>[2x]TETTSFLITKFSPDQQNLIFQGDGYTTKEKLTLTKAVKNTVGRALYSSPIHIWDRETGNVANFVTSFTFVINAPNSYNVADGFTFFIAP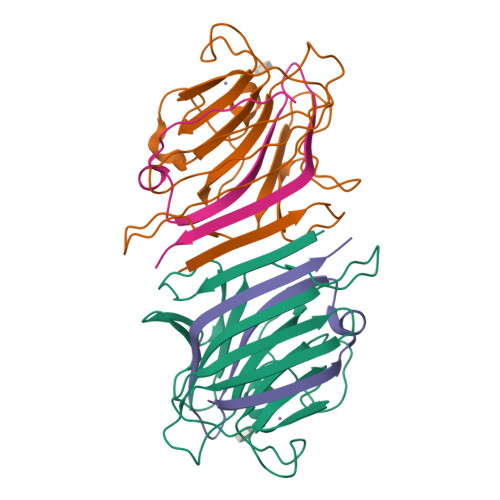VDTKPQTGGGYLGVFNSAEYDKTTQTVAVEFDTFYNAAWDPSNRDRHIGIDVNSIKSVNTKSWKLQNGEEANVVIAFNAATNVLTVSLTYPN;>[2x]VTSYTLSDVVSLKDVVPEWVRIGFSATTGAEYAAHEVLSWSFHSELSGTSSS Maddinglicin A (MadA) produced by Clostridum maddingley belongs to a group of antimicrobial peptides, the so-called lantibiotics or in brief LanA1. The first necessary step is the dehydration of serine and threonine residues, which is catalyzed by the MadB enzyme in the case of MadA. The structure of MadB in the apo-state was determined at an overall resolution of 2.7 Å. MadB is composed of an N-terminal glutamylation (residues 1–741) and a C-terminal elimination (residues 742–1038) domain (see Fig. S1 for the sequence). MadB forms a homodimer as already demonstrated by SEC-MALS with a bifurcate cleft-like structure in the center.

Similarly, for NisB a RMSD of 2.6 Å for 1383 Cα atoms was determined. This indicates that the structure of apo MadB adopts a conformation in between the apo structure of MibB and the substrate-bound structure of NisB. In the apo state, the regulatory loop is stabilized by hydrophobic interactions with Ser154, Glu230, Tyr518, Ser521, and Phe542 as well as hydrogen bonds between the hydroxyl group of Ser180 and Glu178 (distance of 2.7 Å) and between the side chain and backbone of Arg229 with the backbone of Thr168 (distance of 3 Å) and the side chain of Thr168 (distance of 2.7 Å). Surprisingly, the comparison of the apo- and bound-state of MadB revealed a RMSD of 0.2 Å for 1792 Cα atom. The only change occurred in the vicinity of the substrate binding site. More precisely, a loop formed by residues 164–179 had to rotate by 8° to free space for substrate binding, while other minor conformational changes of MadB were located in surface-exposed areas of the protein (see Fig. 5 as well as Movies S1 and S2) and are likely not relevant for catalysis. Interestingly, only at one side of the apo-MadB dimer a tunnel of the GDs envelope was evident. The tunnel is protruding towards the corresponding ED of a monomer indicating that space is present for substrate binding.

>MRDLYRNTNTFMIRTPIFSIDNYYEFFRKDGESDKIKDRLLEICNNSVFREAILVSSKSLYSTIIDFCDGKEIKKFDYFLQSIYKYLIRMSMRPTPFGLFSGVDFGKYAEETVISYENDNFKKFARPDLEWIIKIVKELEDNHYKNLTFKINDSIFIKGERALLIHSTDKEDNNRIGEISIRATKPFMRTYDLAKDGIEYNKLKYILIDEYSIEDESKIDNFLKQLIEREFLISNLRPPLTVLDQFDYLINEVKKAEIEIPLVDELTEIKEKLKLYNETPVGAGEETYLELYKKMESVANVKNILQVDMKLNLRDKKINKKIISDVNDLMNILLDLSMSIENPEPFLSKYKQEFIEKYGQDREISLLEMLDNDIGIGPPMNYERPRNNRSLDVSVNELLDNNVRDYFMEKYFQALKTNSRNIAIRDDEIKNLELQKIDYENIPDSLEINLLVKNKSEDNLSDEFQYYIGPNLGSTSAGKSFGRFSHMMSEPKKFFEELDERNIELIDSEEYVTCEISYLPSEVRNANVTRNIHSSEYEMSLFTNGSKDNLYRIKLNDIYIGLENNTFYAKSKTLNKKLLLTINNMLNPQTAPNAIRFLNDISLDEKKLWYKFVWSDVYKDFSYIPAIKYKNFVIMPETWKMNKINMKINKKTEFNEFKNQFNDYRIKYGVPQYVYITFADNRILLNLDDEQCVKILYHECKNSFNEIILNSYEEEGVNIVKESHKDYICELVIPLTKIKQETISDKVSARMLSSDISSLSKERVKDPFDEWLYIKLYGISSNVDDLIAYYISEFCNELVEEEIISKYFFMRYVDPEQHIRLRLNSSQEKLLMIYPKIREWLSMIRKKGLMTYFSIDSYDREIERYGGIELINIAEKVFFFDSIVTEDILRAKREGSFDFCDEIIGMISVVHYMESFGLPYAKQVEFLRSQVSSSEYREDFKQKRTEYMKLCNSNKDWEGLRESEEGNILIEILNKRRKIIEYYGNKVRENEEVSTDLSILDSIIHLNCNRMFGIDREFEKKVRALASHALYALKHFKS[2x]> GGIQMPVFHTRTIESILEPVAQQISHLVIMHEEGEVDGKAIPDLTAPVSAVQ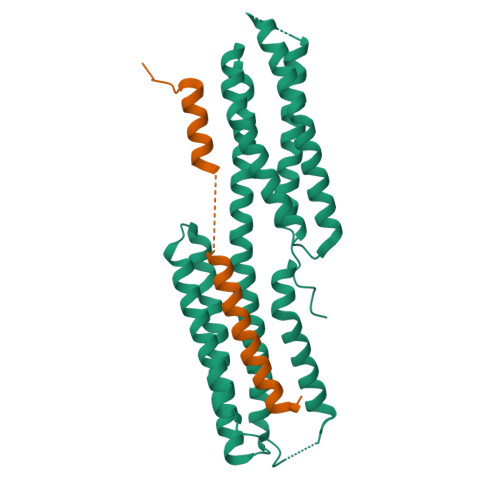AAVSNLVRVGKETVQTTEDQILKRDMPPAFIKVENACTKLVRAAQMLQADPYSVPARDYLIDGSRGILSGTSDLLLTFDEAEVRKIIRVCKGILEYLTVAEVVETMEDLVTYTKNLGPGMTKMAKMIDERQQELTHQEHRVMLVNSMNTVKELLPVLISAMKIFVTTKNTKSQGIEEALKNRNFTVEKMSAEINEIIRVLQLTSWDEDAWA;> GGIQRPSLEERLESIISGAALMADSSCTRDDRRERIVAECNAVRQALQDLLSEYMGNAG> CTTNNLQVTYPAPVAADGWEYRLISTGLTAPRSIVFDSTGGLLVLDAGVGVRRLTLQDNGGTCLSVTANATLIADTALNHGLAISADGGTIYASTVNDVYAYTYNEQTNTVDPTTRRTVVTNMTNTDHVTRTLLLSSRLPNELLVSRGSAANEDPQARNVTSGHSQIRAYDISTLAATDPPFDFVAGTLIGWGLRDSVGVGENPTNGGIWSVENSVDDLTREGVDVHQDNPGEELNFHGILGNTANQGGNYGYPDCYALWSTAGFPDLGALEVGDQFAS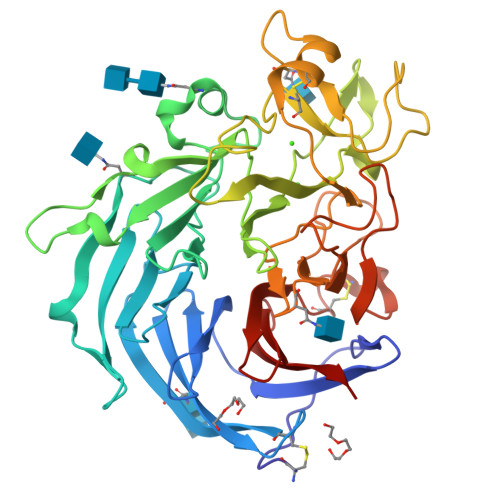DNATAGVTDATCNTNFVDPRLVFQAHVSPLDIKFNTNGTTAYITFHGSTDRTTPVGYSIVSVAFGLNGQPTSPMDSTTAANNILTSPDLTQCPDDCFTPVGLTFDTIGRLFFSSDSTGEIFVLQQS> KTLVSMPPLPGLD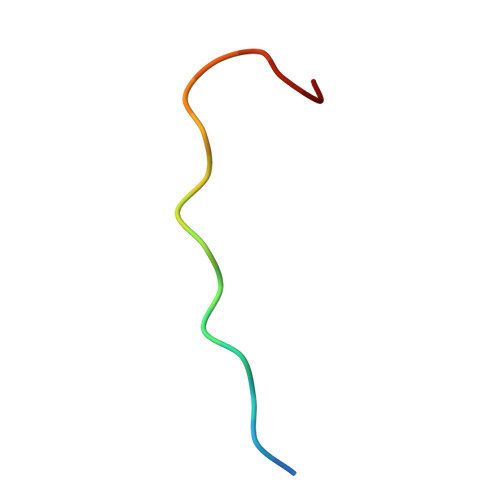LKGS> QCASSPCQNGGSCKDQLQSYICFCLPAFEGRNCETHKDDQLICVNENGGCEQYCSDH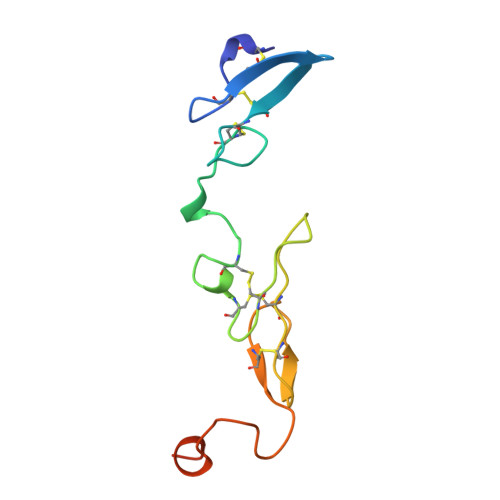TGTKRSCRCHEGYSLLADGVSCTPTVEYPCGKIPILEKRNASKPQGR> MYGDLGNKLVLEAKRTKQLYARSNQDVNLPMYHEDIIRNILKEVSNLRKNTEYLKEQQQLGMLDDKVAKCQYFVTLLCMERNKRCLLAYQRLRTDILDSMAWNNNGLDLMSSITFS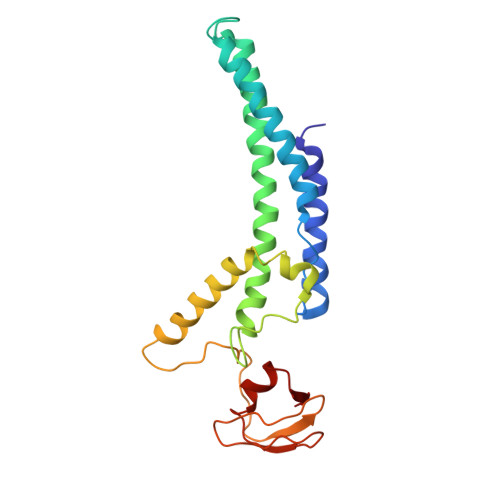QQDTNNLSHQEQEYLKEYCDLITDLKSGDLVDIDLSGSLVPPSDVFIDVRVLKDAGEIQTEYGVFNLIKDSQFFVRQSDVERLIQQGYLQKI>[2x]EYGDLHLFGPNQRPAPCYDPCEAVLVESIPEGLDFPNASTGNPSTSQAWLGLLAGAHSSLDIASFYWTLTNNDTHTQEPSAQQGEEVLRQLQTLAPKGVNVRIAVSKPSGPQPQADLQALLQSGAQVRMVDMQKLTHGVLATKFWVVDQTHFYLGSANMDWRSLTQVKELGVVMYNCSCLARDLTKIFEAYWFLGQAGSSIPSTWPRFYDTRYNQETPMEICLNGTPALAYLASA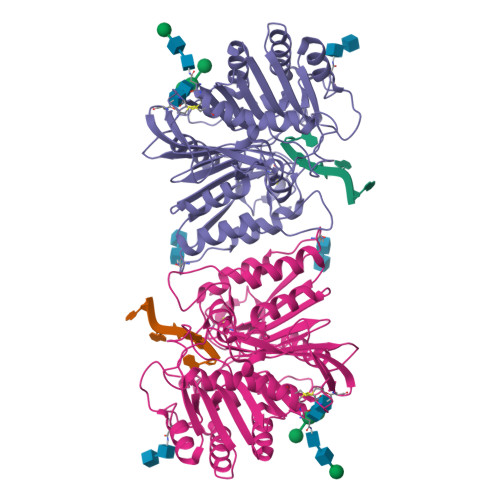PPPLCPSGRTPDLKALLNVVDNARSFIYVAVMNYLPTLEFSHPHRFWPAIDDGLRRATYERGVKVRLLISCWGHSEPSMRAFLLSLAALRDNHTHSDIQVKLFVVPADEAQARIPYARVNANKYMVTERATYIGTSNWSGNYFTETAGTSLLVTQNGRGGLRSQLEAIFLRDWDSPYSHDLDTSADSVGNACRLLLEVLFQ Zearalenone (ZEN) is a mycoestrogenic polyketide produced by Fusarium graminearum and other phytopathogenic members of the genus Fusarium. ZenA cleaves zearalenone [ZEN, (S,E)-14,16-dihydroxy-3-methyl-3,4,5,6,9,10-hexahydro-1H-benzo[c][1]oxacyclotetradecine-1,7(8H)-dione] to hydrolyzed zearalenone [HZEN, (S,E)-2,4-dihydroxy-6-(10-hydroxy-6-oxoundec-1-en-1-yl)benzoic acid], which decarboxylates spontaneously to decarboxylated hydrolyzed zearalenone [DHZEN, (S,E)-1-(3,5-dihydroxyphenyl)-10-hydroxyundec-1-en-6-one]. Furthermore, we report site-directed mutagenesis as well as structural analysis of the dimeric ZenARe of R. erythropolis and the more thermostable, tetrameric ZenAScfl of Streptomyces coelicoflavus with and without bound ligands. The X-ray crystal structures not only revealed canonical features of α/β hydrolases with a cap domain including a Ser-His-Asp catalytic triad but also unusual features including an uncommon oxyanion hole motif and a peripheral, short antiparallel β-sheet involved in tetramer interactions.

For ZenARe, the calculated molar mass of the 6xHis-tagged subunit is 37.103 g/mol (assuming cleavage of the N-terminal fMet), and the observed molar mass of 71 kDa indicated the presence of a dimer. Crystals of space group C 2 2 21 with 2 subunits in the asymmetric unit and 46% solvent content, yielded a dataset of 1.46 Å resolution. The structure was solved by molecular replacement, with ZenAScfl as a search model. The structures of ZenARe and ZenAScfl were found to be very similar, with a RMSD of 0.43 Å (over 502 equiv Cα atoms), with the catalytic triad and oxyanion hole residues superimposing almost perfectly. Most differences between the structures are related to the cap domains. Similar to ZenAScfl, ZenARe shows mostly negative electrostatic surface potential, especially at the active site. While ZenARe has a similar dimeric interface, composed of 30 residues over an interface area of 1195 Å2 (ΔG = −9.4 kcal mol–1, KD = 0.13 μM at 25 °C, according to Prodigy), six amino acids are different in the region corresponding to the tetramer forming interfaces between subunits A/C of ZenAScfl and five amino acids are different in the interface region between the subunits A/D. These differences lead to the abrogation of tetramer stabilizing interactions and corroborate the SEC-MALS result, which showed that ZenARe is a dimer in solution. The catalytic triad of ZenARe was therefore defined as Ser-128 – His-303 – Asp-153.

>[2x]MAEEGTRSEAADAATQARQLPDSRNIFVSHRFPERQVDLGEVVMNFAEAGSPDNPALLLLPEQTGSWWSYEPVMGLLAENFHVFAVDIRGQGRSTWTPRRYSLDNFGNDLVRFIALVIKRPVVVAGNSSGGLLAAWLSAYAMPGQIRAALCEDAPFFASELVPAYGHSVLQAAGPAFELYRDFLGDQWSIGDWKGFVEAAKASPAKAMQLFPTPDEAPQNLKEYDPEWGRAFFEGTVALHCPHDRMLSQVKTPILITHHARTIDPETGELLGALSDLQAEHAQDIIRSAGVRVDYQSHPDALHMMHLFDPARYAEILTSWSATLPANDHHHH> SGVDDDMACHKIPVEADFLYAYSTAPGYYSWRNSKDGSWFIQSLCAMLKQYADKLEFMHILTRVNRKVATEFESFSFDATF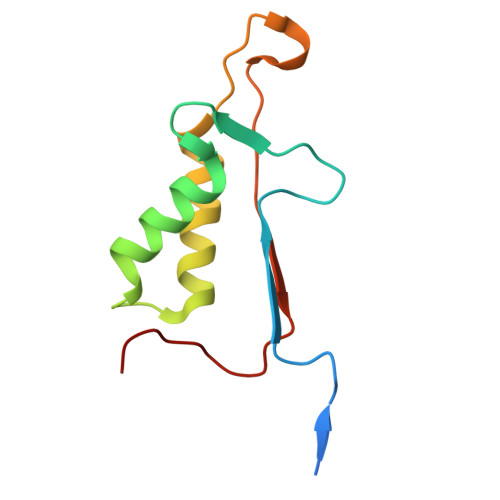HAKKQIPCIVSMLTKELYFYH>[2x]GIQGLAKLIADVAPSAIRENDIKSYFGRKVAIDASMSIYQFLIAVRQGGDVLQNEEGETTSHLMGMFYRTIRMMENGIKPVYVFDGKPPQLKSGELAKRSERRAEAEKQLQQAQAAGAEQEVEKFTKRLVKVTKQHNDECKHLLSLMGIPYLDAPSEAEASCAALVKA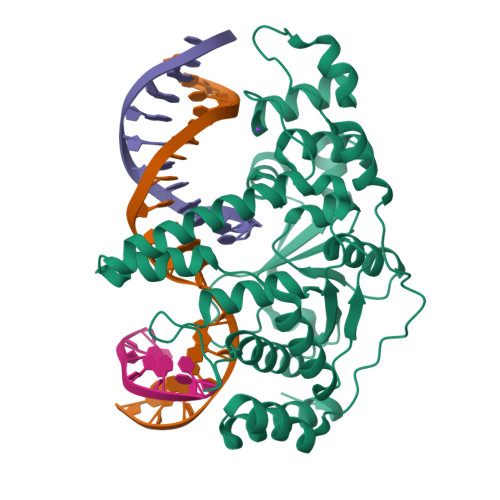GKVYAAATEDMACLTFGSPVLMRHLTASEAKKLPIQEFHLSRILQELGLNQEQFVDLCILLGSDYCESIRGIGPKRAVDLIQKHKSIEEIVRRLDPNKYPVPENWLHKEAHQLFLEPEVLDPESVELKWSEPNEEELIKFMCGEKQFSEERIRSGVKRLSKSRQGSTLEVLFQ> MAQIVDVYGNPIRTQQLREPQTSRLAGLAKEFAQHPAKGLTPAKLARILVEAEQGNLQAQAELFMDMEERDAHLFAEMSKRKRAILGLDWAVEPPRNASAAEKADADYLHELLLDLEGLEDLLLDALDGIGHGYSCIELEWALQGREWMPLAFHHRPQSWFQLNPEDQNELRLRDNSPAGEALQPFGWIIHRPRARSGYVARSGLFRVLAWPYLFRHYATSDLAEML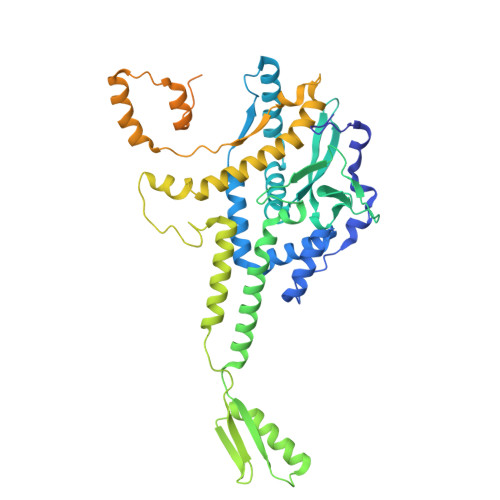EIYGLPIRLGKYPPGTADEEKATLLRAVTGLGHAAAGIIPETMAIDFQQAAQGSSDPFLAMMRQSEDAISKAVLGGTLTSTTSQSGGGAFALGQVHNEVRHDLLASDARQLAATLSRDLLWPLLVLNRPGSPDVRRAPRLVFDLREQADITSMAQSIPALVNVGLEIPSAWVYDKLGIPQPAKNEPVLRSAAQPAILSRQHGQRVAALATIVGPRYGDQQALDKALASLPAKDMQDQVNDLLAPLLEAVNRGDSETELLGALAEAFPDMDDSALTDALHRLLFAADTWGRLHGNLDRID> GAMDPEFELQDGGWSHWS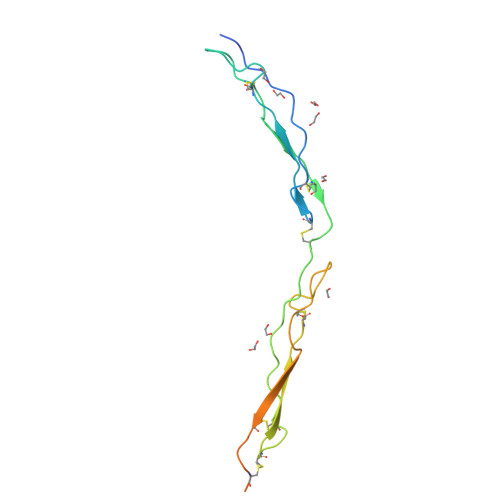PWSSCSVTCGDGVITRIRLCNSPSPQMNGKPCEGEARETKACKKDACPINGGWGPWSPWDICSVTCGGGVQKRSRLCNNPTPQFGGKDCVGDVTENQICNKQDCPLEPYTYRVRFLAKENVTQDAEDNTVSFLQP2,6-dichlorophenol 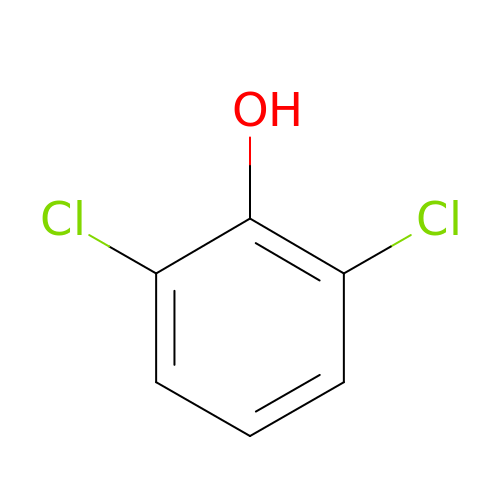| C6 H4 Cl2 O | HOLHYSJJBXSLMV-UHFFFAOYSA-N> SRKLILFIVFLALLLDNMLLTVVVPIIPSYLYSIKHEKNATEIQTARPVHTASISDSFQSIFSYYDNSTMVTGNATRDLTLHQ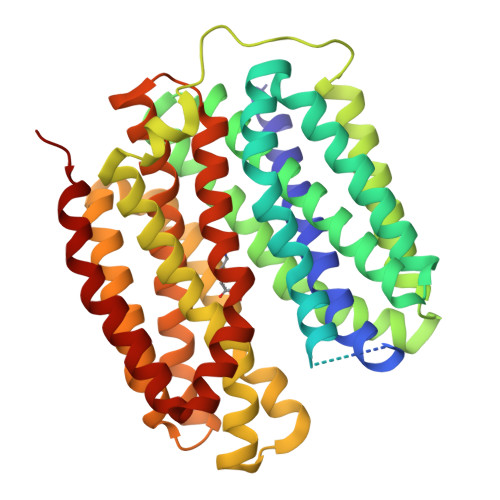TATQHMVTNASAVPSDCPSEDKDLLNENVQVGLLFASKATVQLITNPFIGLLTNRIGYPIPIFAGFCIMFVSTIMFAFSSSYAFLLIARSLQGIGSSCSSVAGMGMLASVYTDDEERGNVMGIALGGLAMGVLVGPPFGSVLYEFVGKTAPFLVLAALVLLDGAIQLFVLQPSRVQPESQKGTPLTTLLKDPYILIAAGSICFANMGIAMLEPALPIWMMETMCSRKWQLGVAFLPASISYLIGTNIFGILAHKMGRWLCALLGMIIVGVSILCIPFAKNIYGLIAPNFGVGFAIGMVDSSMMPIMGYLVDLRHVSVYGSVYAIADVAFCMGYAIGPSAGGAIAKAIGFPWLMTIIGIIDILFAPLCFFLRSPP4-[(2~{R})-2-carboxy-5-(oxidanylamino)-5-oxidanylidene-pentyl]benzoic acid | C13 H15 N O6 | 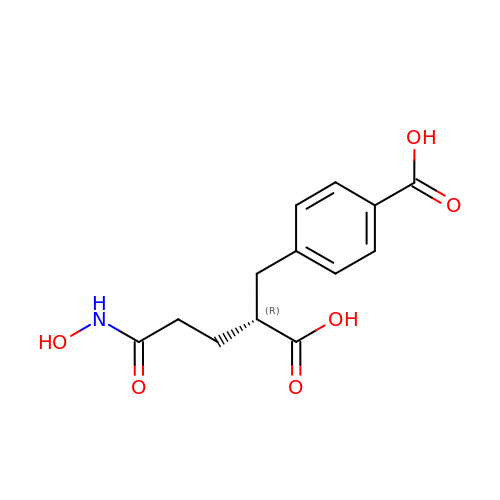VUDGMYIWOPKVSL-SNVBAGLBSA-N> EATECLTRSNLKKLQEKIFDRELNDIACDHCLCSTENRRDIKYSRLW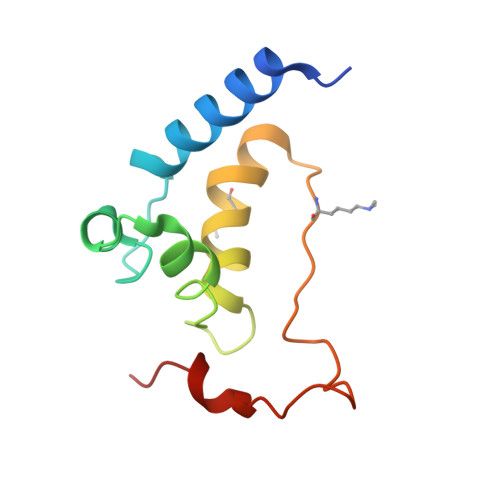FLFELEMSENWNENLRLSCYNKYVYSAIDESWKMENILLKEQEKHYEYFPIGQLLIPN>[2x]HHHHHHFNLPPGNYKKPKLLYCSNGGHFLRILPDGTVDGTRDRSDQHIQLQLSAESVGEVYIKSTETGQYLAMDTDGLL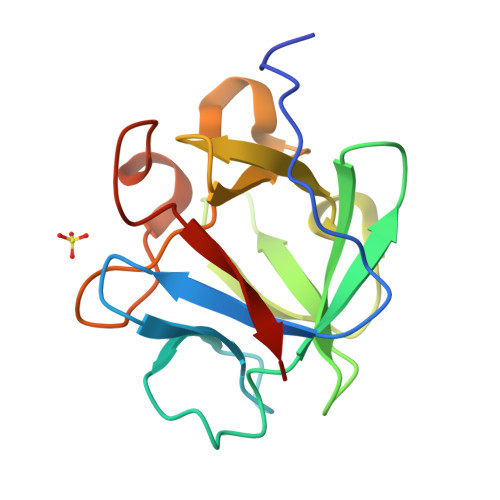YGSQTPNANCLFLERLEENHYNTYISKAHAEKNWFVGLKKNGSCKRGPRTHYGQKAILFLPLPVSSD>QLTTESMPFNVAEGKEVLLLVHNLPQQLFGYSWYKGERVDGNRQIVGYAIGTQQATPGPANSGRETIYPNASLLIQNVTQNDTGFYTLQVIKSDLVAEEA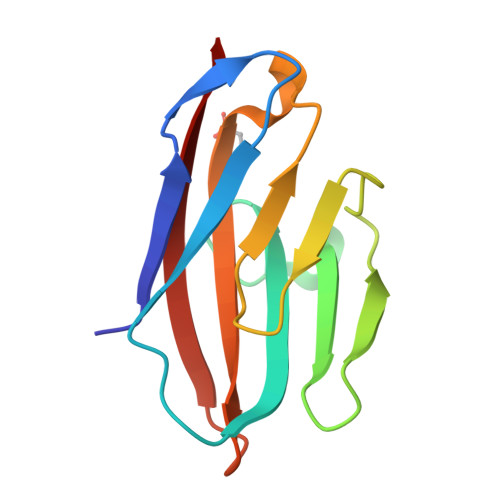TGQFHVY[2x]> MRGSHHHHHHGSACCASRDDWRCARSMHEFSAKDIDGHMVNLDKYRGFVCIVTNVASQCGKTEVNYTQLVDLHARYAECGLRILAFPCNQFGKQEPGSNEEIKEFAAGYNVKFDMFSKICVNGDDAHPLWKWMKIQ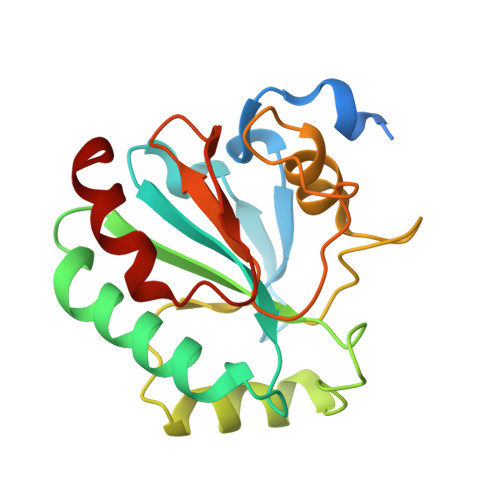PKGKGILGNAIKWNFTKFLIDKNGCVVKRYGPMEEPLVIEKDLPHYF>MPVTDVKHDLDTLTLTITAEFAAPVTRIWQIYADPRQLEKVWGPPSHPATVVDHDLRPGGRVTYFMTGPDGEKYAGYWEITAVDEPHSF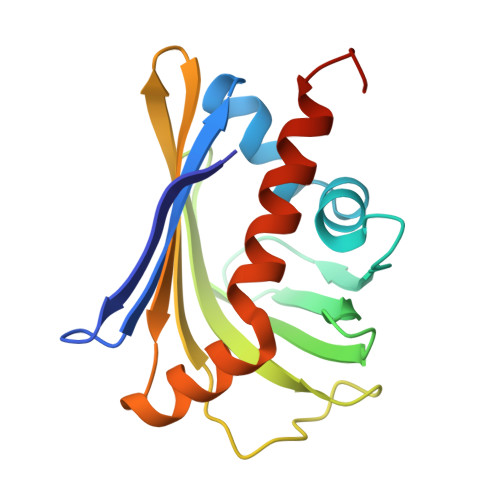SFLDGFADEDFNPNTDLPVSTNVYTFTEHDGGTRATYVGTYASAEALQQVLDMGVIEGASSAINQIDALLTATHHHHHH[2x]> SRKKRKRCGTCDPCRRLENCGSCTSCT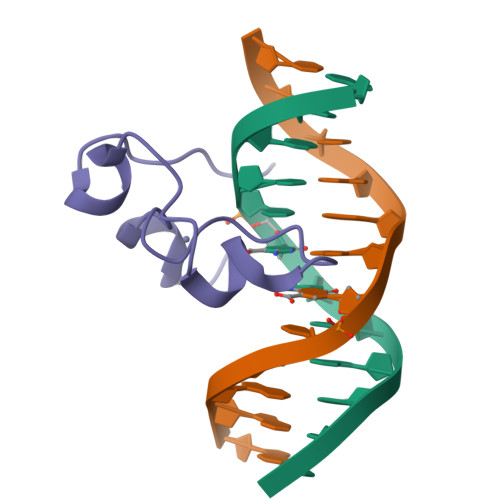NRRTHQICKLRKCEVLKKKA>RRGSFVEMVDNLRGKSGQGYYVEMTVGSPPQTLNILVDTGSSNFAVGAAPHPFLHRYYQRQLSSTYRDLRKGVYVPYTQGKWEGELGTDLVSIPHGPNVTVRANIAAITESDKFFINGSNWEGILGLAYAEIARPDDSLEPFFDSLVKQTHVPNLFSLQLCGAGFPLNQSEVLASVGGSMIIGGIDHSLYTGSLWYTPIRREWYYEVIIVRVEINGQDLKMDCKEYNYDKSIVDSGTTNLRLPKKVFEAAVKSIKAASSTEKFPDGFWLGEQLVCWQAGTTPWNIFPVISLYLMGEVTNQSFRITILPQQYLRPVE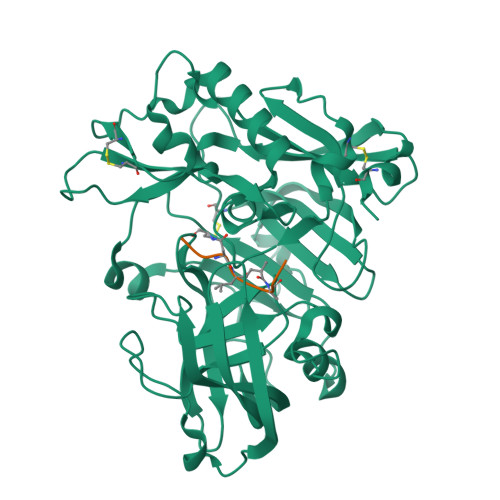DVATSQDDCYKFAISQSSTGTVMGAVIMEGFYVVFDRARKRIGFAVSACHVHDEFRTAAVEGPFVTLDMEDCGYN[2x];>[2x]EVNXAEF3-[2,6-bis(oxidanylidene)-4-(trifluoromethyl)-5~{H}-pyrimidin-1-yl]-~{N}-methyl-2-pyridin-2-yl-imidazo[1,2-a]pyridine-7-carboxamide 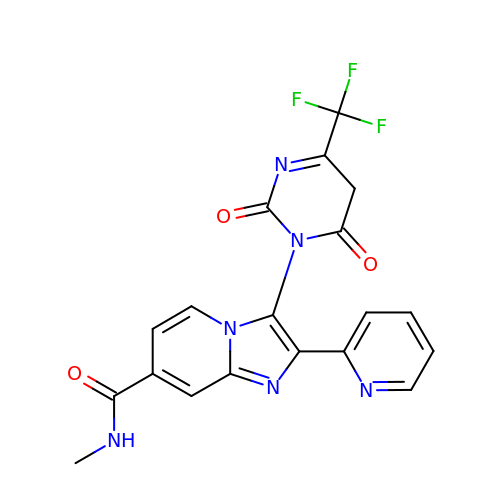| C19 H13 F3 N6 O3 | QORQCYPXGXBYBR-UHFFFAOYSA-N> PPGP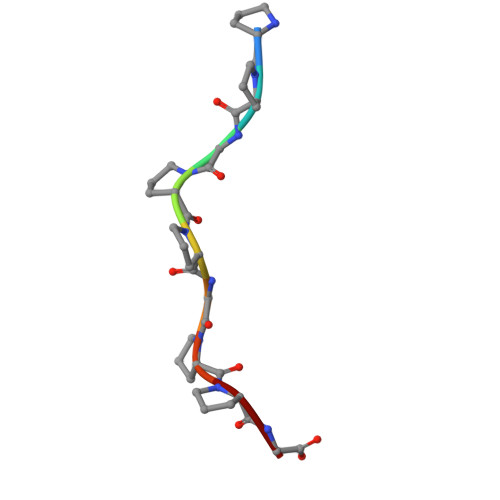PGPPG>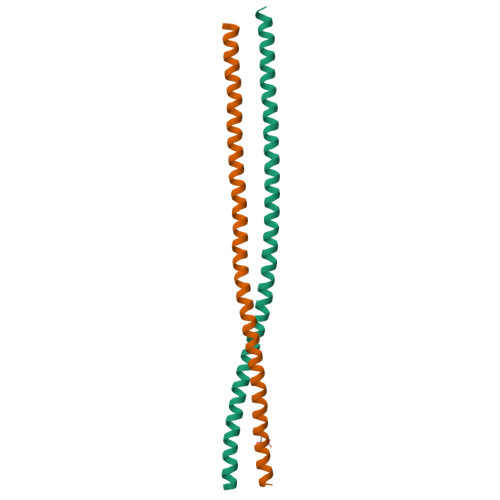GSSLQRYEKLVKECRRLEEELEQKTHEASDASQRVRQLERETTRLMRRVEQLVSAVEGQKQKLDETEAKHKLELAEIENRHELEIQSKMSSHEEALRRLMDARR[2x]1-biphenyl-2-ylmethanamine 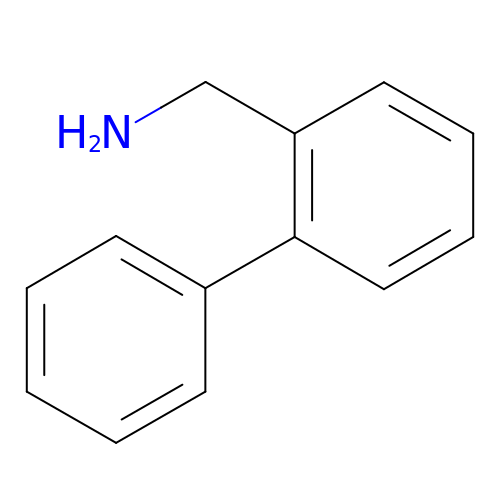| C13 H13 N | YHXKXVFQHWJYOD-UHFFFAOYSA-N> GPLGSMSSMNPEYDYLFKLLLIGDSGVGKSCLLLRFADDTYTESYISTIGVDFKIRTIELDGKTIKLQIWDTAGQERFRTITSSYYRGAHGIIVVYDVTDQESFNNVKQWLQEIDRYASENVNKLLVGNKCDLTTKKVVDYTTAKEFADSLGIPFLETSAKNATNVEQSFMTMAAEIKKRMGPGATAGGAEKSNVK;> GPLGSTSSTSQADKEIQKMLDEYEQAIKRAQENIKKGEELEKKLDKLERQGKDLEDKYKTYEE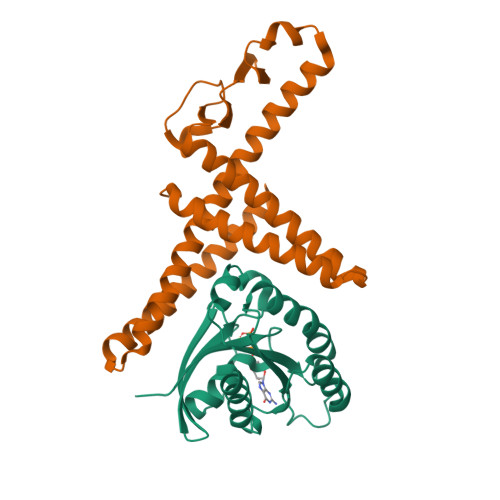NLEGFEKLLTDSEELSLSEINEKMKAFSKDSEKLTQLMEKHKGDEKTVQSLQREHHDIKAKLANLQVLHDAHTGKKSYVNEKGNPVSSLKDAHLAINKDQEVVEHKGQFYLLQKGQWDAIKNDPAALEKAQKDYSQSKHDLATIKMEALIHKLSLEMEKQLETINDLIMSTDPKENEEATKLLHKHNGLNLKLANLQDMLAVHR>[2x]GMVNPISRLMQIQQARKEK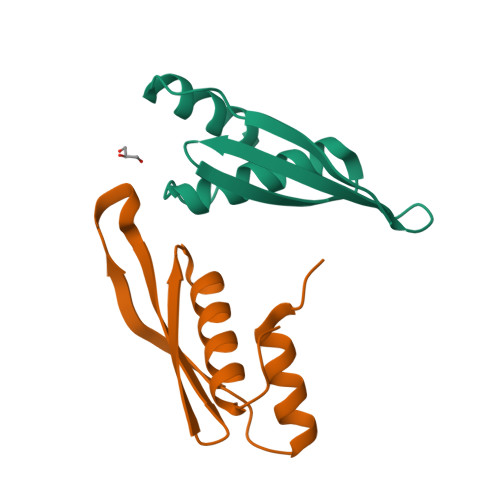EPVYTLVEERGVARRREFIMEVSASGKSATGIGPTKKLAKKEAAENLLVMLGYGRS>STAGKVIKCKAAVLWEVKKPFSIEDVEVAPPKAYEVRIKMVAVG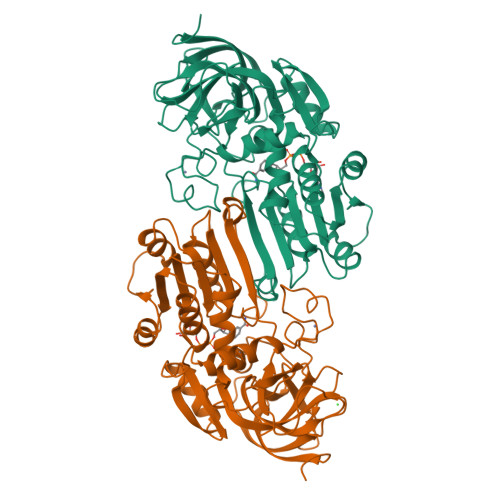ICGTDDHVVSGNLVTPLPVILGHEAAGIVESVGEGVTTVKPGDKVIPLFTPQCGKCRVCKNPESNYCLKNDLGNPRGTLQDGTRRFTCRGKPIHHFLGTSTFSQYTVVDENAVAKIDAASPLEKVCLIGCGFSTGYGSAVNVAKVTPGSTCAVFGLGGVGLSAVMGCKAAGAARIIAVDINKDKFAKAKELGATECINPQDYKKPIQEVLKEMTDGGVDFSFEVIGRLDTMMASLLCCHEACGTSVIVGVPPASQNLSINPMLLLTGRTWKGAVYGGFKSKEGIPKLVADFMAKKFSLDALITHVLPFEKINEGFDLLHSGKSIRTVLTF[2x]>[2x]MDEFEMIKRNTSEIISEEELREVLKKDEKSAGIGFEPSGKIHLGHYLQIKKMIDLQNAGFDIIIGLADLHAYLNQKGELDEIRKIGDYNKKVFEAMGLKAKYVYGSEEQLDKDYTLNVYRLALKTTLKRARRSMELIAREDENPKVAEVIYPIMQVNSIHYEGVDVAVGGMEQRKIHMLARELLPKKVVCIHNPVLTGLDGEGKMSSSKGNFIAVDDSPEEIRAKIKKAYCPAGVVEGNPIMEIAKYFLEYPLTIKRPEKFGGDLTVNSYEELESLFKNKELHPMRLKNAVAEELIKILEPIRKRLSDPENLYFQ

Genetically encoded caged amino acids can be used to control the dynamics of protein activities and cellular localization in response to external cues. In the present study, we revealed the structural basis for the recognition of O-(2-nitrobenzyl)-L-tyrosine (oNBTyr) by its specific variant of Methanocaldococcus jannaschii tyrosyl-tRNA synthetase (oNBTyrRS), and then demonstrated its potential availability for time-resolved X-ray crystallography. In contrast, the genetic encoding of caged amino acids offers a more facile and robust approach for biosynthesizing the photoresponsive proteins. These synthetic amino acids are recognized by specific variants of aminoacyl-tRNA synthetase and attach to tRNA, which in turn translates codons (mostly the UAG stop codon) assigned to the amino acids. Thus, cell-free protein synthesis of caged proteins with oNBTyr could facilitate time-resolved structural analysis of proteins, including medically important membrane proteins.

In the present study, we determined the crystal structure of another archaeal tyrosyl-tRNA synthetase variant (oNBTyrRS) complexed with O-(2-nitrobenzyl)-L-tyrosine. The substrate-bound crystal structure of oNBTyrRS at a 2.79 Å resolution indicated that the replacement of tyrosine and leucine at positions 32 and 65 by glycine (Tyr32Gly and Leu65Gly, respectively) and Asp158Ser created sufficient space for entry of the bulky substitute into the amino acid binding pocket, while Glu in place of Leu162 formed a hydrogen bond with the nitro moiety of oNBTyr. The five mutated residues play essential roles in the recognition of the structural features of oNBTyr. The substitutions of Tyr32 and Leu65 for Gly and Asp158 for Ser created enough space to accommodate the bulky nitrobenzyl group. In addition, glutamates replaced with Phe108 and Leu162 form a so-called carboxyl (Glu108)-carboxylate (Glu162) dimer motif. Furthermore, these residues, together with the oxygen of the nitro group, formed a hydrogen-bonding network, which was stabilized by the participation of Ser158. The nitro group was slightly bent with respect to the planarity of the benzyl group, thus the crucial recognition of the nitro group, which is important for substrate discrimination, was exhibited. Although the chemical structure of oNPTyr was larger than that of oNBTyr, the fitting model showed no structural distortion. This is because the substrate binding pocket of oNBTyrRS was open toward the surface of the enzyme. The nitro group of the leaving group forms a polar interaction only with the main chain of Ala70 in the hydrophobic environment. These comparisons indicate that two different mechanisms are achieved among the synthetase variants for the recognition of the same leaving group. It provides a structural basis for the recognition of caged tyrosine, oNBTyr by mutant TyrRS.> QEFHFGPCQVKGVVPQKLWEAFWAVKDTMQAQDQITSARLLQQEVLQQVSDAESCYLVHTLLEFYLKTVFKNHHQRTVEVRTLKSFSTLANNFVLIVSQLQPSQENEMFSIRDSAHRRFLLFRRAFKQLDVEAALTKALGEVDILLTWMQKFYKL;> LPAPQNLSVLSTNMKHLLMWSPVIAPGETVYYSVEYQGEYESLYTSHIWIPSSWCSLTE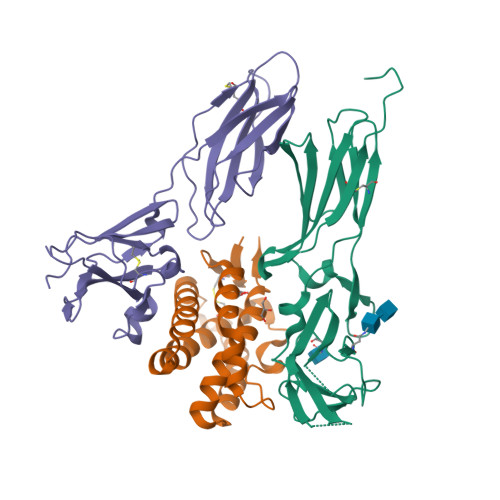GPECDVTDDITATVPYNLRVRATLGSQTSAWSILKHPFNRQSTILTRPGMEITKDGFHLVIELEDLGPQFEFLVAYWRREPGAEEHVKMVRSGGIPVHLETMEPGAAYCVKAETFVKAIGRYSAFSQTECV;> LLQHVKFQSSNFENILTWDSGPEGTPDTVYSIEYKTYGERDWVAKKGCQRITRKSCNLTVETGNLTELYYARVTAVSAGGRSATKMTDRFSSLQHTTLKPPDVTCISKVRSIQMIVHPTPTPIRAGDGHRLTLEDIFHDLFYHLELQVNRTYQMHLGGKQREYEFFGLTPDTEFLGTIMICVPTWAKESAPYMCRVKTLPDRTWTG>[2x]SAAAALRDQLTAL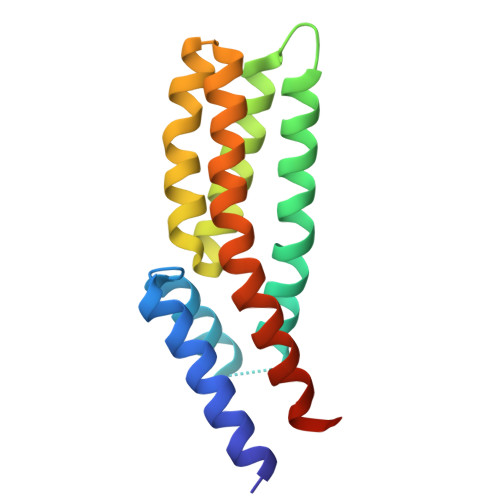LSSMFSQGLVDEQFQQLQMLQDEGGTPGFVSEVVTLFCDDADRIINEIATLLEQPVVNFDKVDAYVHQLKGSSASVGAQKVKFTCMQFRQFCQDKSRDGCLMALAVVRNDFYDLRNKFQTMLQLEQQIQAYDPKQQ> GSAEQVTKSVLFVCLGNICRSPIAEAVFRKLVTDQNISDNWVIDSGAVSDYEVGRSPDPRAVSCLRNHGINTAHKARQVTKEDFVTFDYILCMDESNLRDLNRKSNQVKNCRAKIEL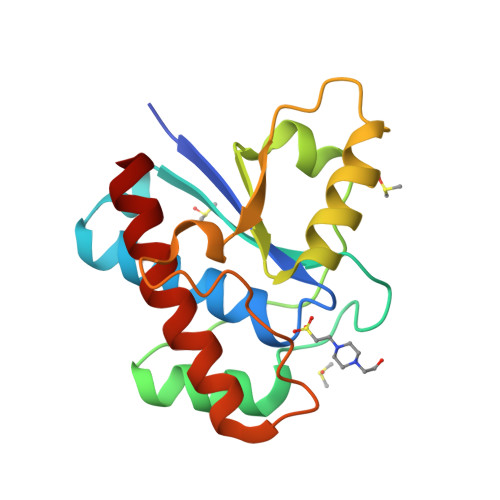LGSYDPQKQLIIEDPYYGNDADFETVYQQCVRCCRAFLEKVR>[6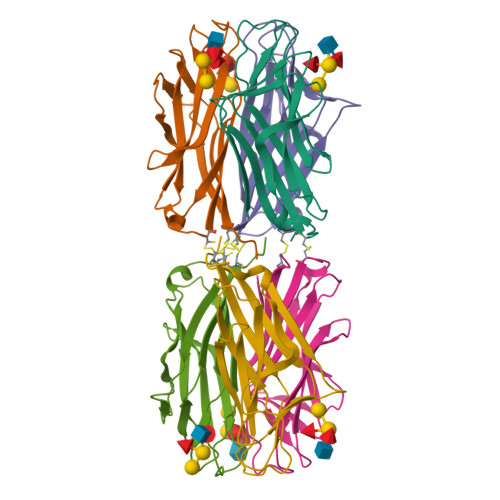x]MSIVFASIDPRSNPLQTSSQNYVDIPGLKLDVSKYSNSPCLTALITLNIPTPYASGNNFPGGNFAIVTDQGEQLAYGGFTYSSKIPENSGRMPFTLVARYSLASNVSTIKAQWSNIRGSTVHIDSYASISAVIQCNQLV>[2x]MTVQMEYEKDVKVAALDGKKIAVIGYGSQGHAHAQNLRDSGRDVIIGVRPGKSFDKAKEDGFDTYTVAEATKLADVIMILAPGEIQQELYEAEIAPNLEAGNAVGFAHGFNIHFEFIKVPADVDVFMCAPKGPGHLVRRTYEE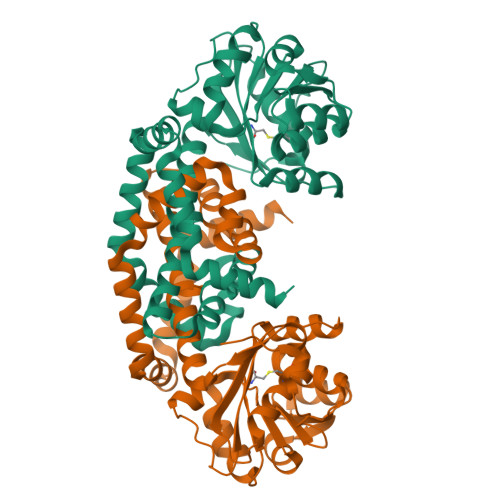GFGVPALYAVYQDATGNAKNIAMDWCKGVGAARVGLLETTYKEETEEDLFGEQAVLCGGLTALIEAGFEVLTEAGYAPELAYFEVLHEMKLIVDLIYEGGFKKMRQSISNTAEYGDYVSGPRVITEQVKENMKAVLADIQNGKFANDFVNDYKAGRPKLTAYREQAANLEIEKVGAELRKAMPFVGKNDDDAFKIYN> QSSKRSSRSVEDDKEGHLVCRIGDWLQERYEIVGNLGEGTFGKVVECLDHARGKSQVALKIIRNVGKYREAARLEINVLKKIKEKDKENKFLCVLMSDWFNFHGHMCIAFELLGKNTFEFLKENNFQPYPLPHVRHMAYQLCHALRFLHENQLTHTDLKPENILFVNSEFETLYNEHKSCE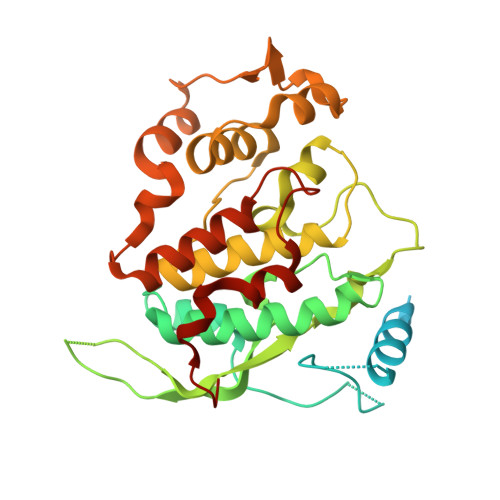EKSVKNTSIRVADFGSATFDHEHHTTIVATRHYRPPEVILELGWAQPCDVWSIGCILFEYYRGFTLFQTHENREHLVMMEKILGPIPSHMIHRTRKQKYFYKGGLVWDENSSDGRYVKENCKPLKSYMLQDSLEHVQLFDLMRRMLEFDPAQRITLAEALLHPFFAGLTPEERSFH>SMPTPEAPYASLTEIEHLVQSVSKSYRETCQLRLEDLLRQRSNIFSREEVTGYQRKSMWEMWERCAHHLTEAIQYVVEFAK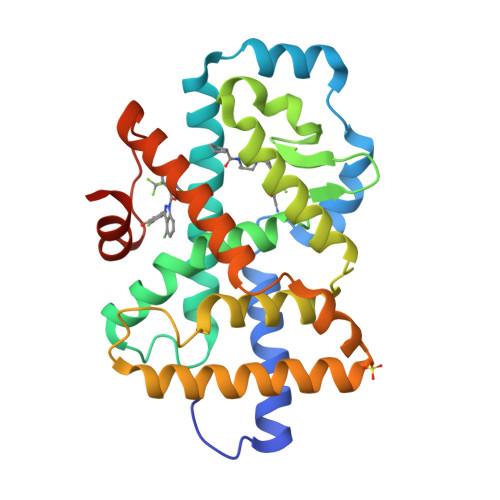RLSGFMELSQNDQIVLLKAGAMEVVLVRMCRAYNADNRTVFFEGKYGGMELFRALGCSELISSIFDFSHSLSALHFSEDEIALYTALVLINAHRPGLQEKRKVEQLQYNLELAFHHHLCKTHRQSILAKLPPKGKLRSLCSQHVERLQIFQHLHPIVVQAAFPPLYKELFSTETESPVGLS[2x]> ERLCHPCPWEWTFFQGNCYFMSNSQRNWHDSITACKEVGAQLVVIKSAEEQNFLQLQSS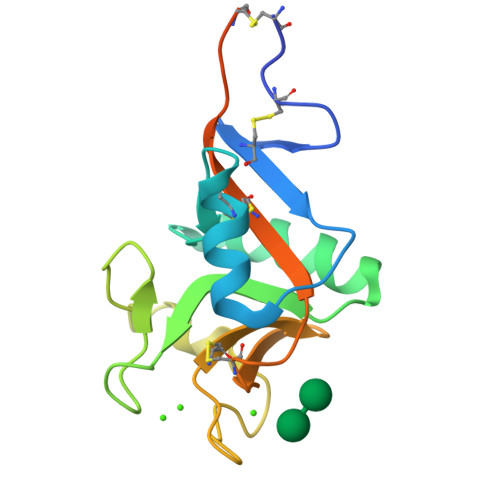RSNRFTWMGLSDLNQEGTWQWVDGSPLLPSFKQYWNRGEPNNVGEEDCAEFSGNGWNDDKCNLAKFWICKKSAASCSRDEEQFLSPAPATPNPPPA>MVVKRTQTDSRMQSTPGNHNHPDAHANAAYMTPPSMGALNANNSNSQLSTLTISPMTYLANNTSTDGSFLKERNAQNTDSLSREDYLRLWRHDALMQQQYKCAAFVGEKVLDITGNPNDAFWLAQVYCCTGDYARAKCLLTKEDLYNRSSACRYLAAFCLVKLYDWQGALNLLGETNPFRKDEKNANKLLMQDGGIKLEASMCYLRGQVYTNLSNFDRAKECYKEALMVDAKCYEAFDQLVSNHLLTADEEWDLVLKLNYSTYSKEDAAFLRSLYMLKLNKTSHEDELRRAEDYLSSINGLEKSSDLLLCKADTLFVRSRFIDVLAITTKILEIDPYNLDVYPLHLASLHESGEKNKLYLISNDLVDRHPEKAVTWLAVGIYYLCVNKISEARRYFSKSSTMDPQFGPAWIGFAHSFAIEGEHDQAISAYTTAARLFQGTHLPYLFLGMQHMQLGNILLANEYLQSSYALFQY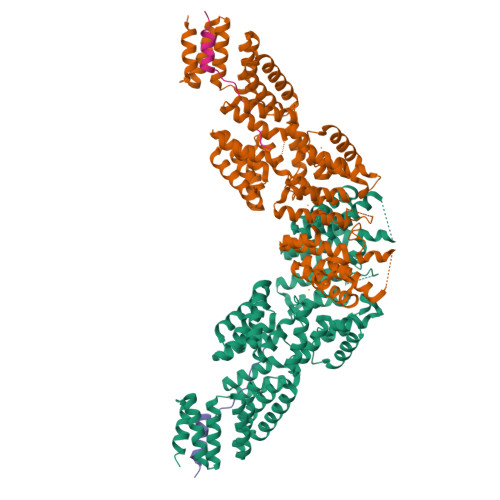DPLLLNELGVVAFNKSDMQTAINHFQNALLLVKKTQSNEKPWAATWANLGHAYRKLKMYDAAIDALNQGLLLSTNDANVHTAIALVYLHKKIPGLAITHLHESLAISPNEIMASDLLKRALEEN[2x];>[2x]XMLRRNPTAIQITAEDVLAYDEEKLRQTLDSESTTEEALQKNEESTRLSPEKKKIIRERRIGITQIFDSSMHPSQGGAAQS> MKKLSRTISGVTPVAVMTKPLPCPGKCIYCPTFAATPQSYTPESPAVLRAKSCEYQAYKQVALRLRIIQDMGHPTDKVELIIMGGTFLSADITYQYGFIKDCYDALNGVVAGSLEEAKTINETAQHRCVGLCIETRPDICGKAEIQRMIDFGTTRVELGVQMLDDDIYKLVERGHRVSDVAEATCLLREYGLKVHYHWMPGLPGSSPEKDLALSRMVFEDPRFCPDGLKLYPTMVVEGTILEQWWKEGRYTPYPNGTMT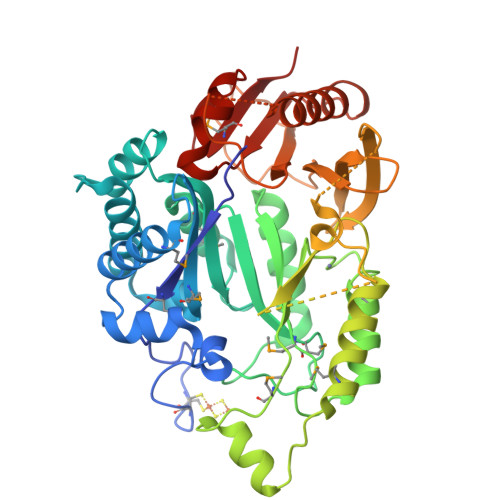GLIADIKALVPPYVRISRVLRDIPAVFISAGLKDSLRDGVRQILESRHQKCRCIRCREYGHRQRKGQTSGEPTLRRLDYPASGGKEIFLSFEDASDTLYGLLRLRIPCASLPVLGQKYGAKTGLVRELHVYGTELSLGEQGDQSAQHRGLGRKLLAEAECLARDEFGLDSLAILSGVGAREYYRSLGYELVAGYMCKHLD> MVTLHLAHLTLTHAQPSYAALECIPAMQRRRLSPLAKLALNTAISSLDGRSADYIVWVSKYGDEAKTLNILQDVLNDQTPSPTQFSTSVHNAISGLYSILCQDDTPSTSLSCSWTEGLIEAYALLKSMPEIKRVLVVAYDEPLPNIYAEAINFPAYAMAAVVTLEQPNLQITAWTHTDEAEAPAFAHF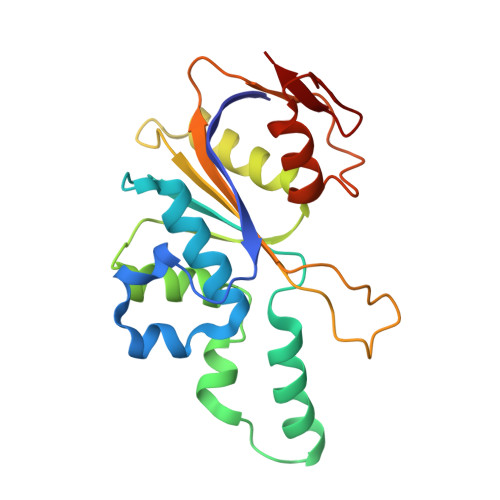WQDADQLTSAFGWNKC>[7x]VFSDFLLKDPPESKYKGLRLELAVDKLVSCIAVGLPLLLISLAFAQEITLGSQISCFAPTSFSWR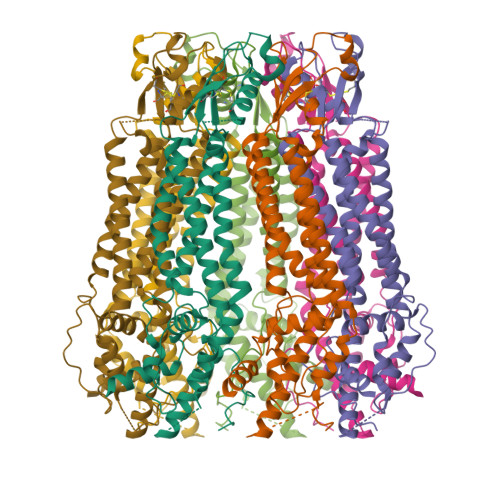QAAYVDSFCWAAVQQKHLSQSDSGNVPLWLHKFFPYILLLVAVLLYLPNLFWRFTAAPHLSSDLKFVMEELDKCYNRDIKDIKAANNLNSSDKRDGLNSPVVSENLQQSLWEIPLSHYKYPIVEQYLKTKNNSYGLIIKYLICRVVTLIIVFTACIYLGYYISLFSLTDEFTCNIRTGILRNDTALPPLVQCKLIAVGVFRLLSYINLIIYVLIMPFIIYAMLVPFRKTANVLKVYEVLPTFSVQQAPSKTYDDHSLFLLFLEENVSELKSYKFLKVLENIK>[2x]ALVIAFIGKNGAVMAGDMREITFEGEKPDREKLEKELYSGSIVTDEEM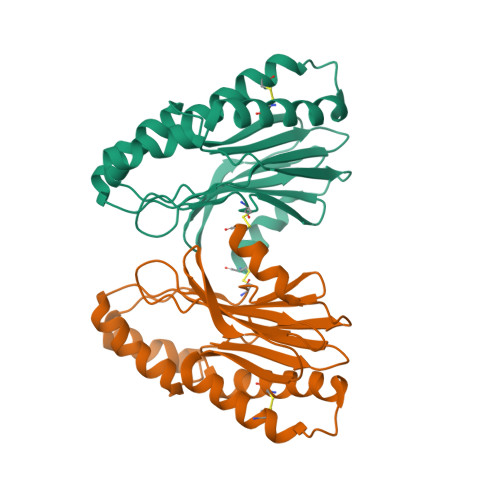QKKAEEFGVKITVADCKEKVSERNGVLVGEVSSAEGGVVKKRRLYASAGNFAIAELINTEMTLTSQGKGSNFIAFGNEFTKQVANKCFKDNWTKKSNLQDAVKILILCMETVARKTASVSKQFMIVQTASNADVLKVVEKDRNC>[2x]GSHMASNDLIYQDEHASLQPLEGRTVAVIGYGIQGRAFAANLRDSGVAVRVGNIDDRYFELARAEGHRVTNIAEAVAHADIVLLLIPDEAHGAVFDVDIAPNLRDGALLCVAHGHSLVQGDVRPLPGRDLAMLAPRMYGDPIRRYYLAGQGAPAYFDIVADHTGRARDRVLAIARAVGFTRAGVMALGYRQETFLDLFQEQFLAPALVDLVETGFQVLVERGFNPKAALLEVYGSGQMGKMMLDGADIGLDEVVALQGSPTCQVGYHRWRGRTLPTAVRELAARVLDQIEGGDFSAYLKEQASNDYASLDDARRAALKRPLNVAHAQVRAAFRFPTEAAGGLYQAAQAPADVEPEAAR

A trait of BP bacteria is a conserved gene cluster coding for the biosynthesis of polyketides (malleicyprols) with a reactive cyclopropanol unit that is critical for virulence. We show that BurG, an unusual NAD+-dependent member of the ketol-acid reductoisomerase family, constructs the strained cyclopropanol ring. A sequence similarity search using BLAST predicted that BurG belongs to the family of ketol-acid reductoisomerases (KARIs; EC 1.1.1.86), well-characterized enzymes that play key roles in the biosynthesis of branched-chain amino acids. Biochemical assays and a suite of eight crystal structures of native and mutated BurG with bound analogues and inhibitors provide snapshots of each step of the complex reaction mechanism, involving a concealed oxidoreduction and a C–S bond cleavage.

Our structural analysis revealed that the carboxylate of a glutamic acid side chain (E232) is in close proximity (3 Å) to the β carbons of the substrate surrogates and thus probably facilitates the deprotonation event necessary for enol formation. To probe the function of this putative catalytic residue we generated a point-mutated variant (E232Q) of BurG and assayed its activity with the native substrate gonydiol. As predicted, the mutation hampers the transformation of gonydiol into the cyclopropanol derivative 6. Co-incubations of BurG E232Q with rac-12 yielded crystals for which we solved a 3D structure at a resolution of 1.55 Å. The absence of oxidized 13 in BurG E232Q may indicate a role of E232 in shifting the internal redox equilibrium towards the oxidized state by deprotonating the substrate and forming the enolate. By analogy to glycerate oxidation, the oxidized state is probably energetically less favoured. The obtained near-atomic resolution structure with BurG E232Q and 12 enabled us to analyse the bound ligand and determine its absolute configuration (2R,3R). The observed chirality of the bound substrate confirmed our stereochemical analysis that gonydiol had the 2R,3R configuration. Intermediate 14 is firmly held in place by ionic interaction of its sulfonium moiety with E232 and cation–π interaction with Y133. In contrast, the neutral carba analogues 12 and 13 show a higher degree of freedom in their tail regions due to the lack of ionic placement as visible in their crystallographic B factor.> NTFEDFYLKRELLMGIFEAGFEKPSPIQEEAIPVAITGRDILARAKNGTGKTAAFVIPTLEKVKPKLNKIQALIMVPTRELALQTSQVVRTLGKHCGISCMVTTGGTNLRDDILRLNETVHILVGTPGRVLDLASRKVADLSDCSLFIMDEADKMLSRDFKTIIEQILSFLPPTHQSLLFSATFPLTVDEFMDKHLHKPYEINLMEELTLKGITQYYAFVEERQKLHCLNTLFSKLQINQAIIFCNSTNRVELLAKKITDLGYSCYYSHARMKQQERNKVFHEFRQGKVRTLVCSDLLTRGIDI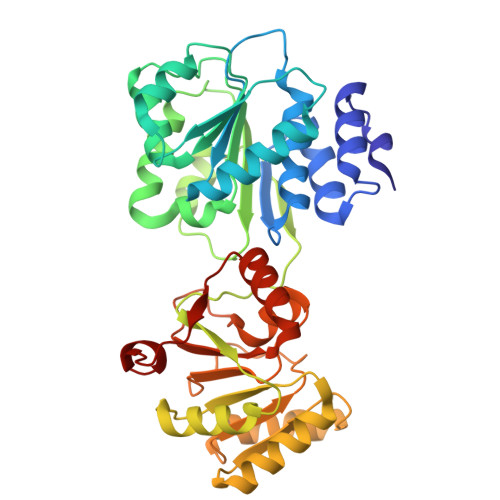QAVNVVINFDFPKTAETYLHRIGRSGRFGHLGLAINLINWNDRFNLYKIEQELGTEIAAIPATIDKSLYVAEN Here, we report the structure and function of the O. tauri photosystem I (PSI) supercomplex in low light conditions, where it expands its photon-absorbing capacity by assembling with the light-harvesting complexes I (LHCI) and a prasinophyte-specific light-harvesting complex (Lhcp). Interestingly, nine Lhcp subunits, including one Lhcp1 monomer with a phosphorylated amino-terminal threonine and eight Lhcp2 monomers, oligomerize into three trimers and associate with PSI on the third side between Lhca6 and PsaK. While Lhcp, Lhcb (apoproteins of LHCII), and Lhca (apoproteins of LHCI) all belong to the LHC superfamily, Lhcp proteins form a separate clade with characteristics of an ancestral state of LHC proteins instead of belonging to the clades of Lhcb or Lhca. In terms of pigment composition, OtLhcp1 and OtLhcp2 each contain 14 Chl molecules (8 Chl a, 5 Chl b, and 1 Mdp) and 7 carotenoid molecules (4 Dlt, 2 Prx, and 1 Nex).

Among the three trimers associated with OtPSI, Trimers 1 and 3 are both (Lhcp2)3 homotrimers, whereas Trimer 2 is a Lhcp1(Lhcp2)2 heterotrimer. Trimers 1 and 3 bind to PSI on the PsaO and PsaK sides, respectively, while Trimer 2 assembles with PSI on the PsaL-PsaH side through Lhcp1 subunit and interacts with Lhca6 through an Lhcp2 subunit. As Trimer 1 is sandwiched between Trimers 2 and 3, it forms close contacts with both Trimers 2 and 3, and is related with them through pseudo-C2 symmetry axes at their interfaces. Among these subunits, Trimers 1 and 2 interact with each other closely and may form a stable hexameric unit. When the PSI core regions are aligned, O. tauri Trimer 1 appears to be rotated by 57 degrees and shifted by 16.1 Å in relation to the position of C. reinhardtii LHCII-1. Trimer 1 is located nearby PsaO and the closest interfacial distances between them are 7.0 Å or larger. Although Trimer 1 does not form direct interactions with PsaO, we cannot rule out the presence of unresolved lipid molecules that may mediate the interactions. In contrast, Trimer 1 appears to be poorly connected with PSI as it has Chl b molecules (Chls b608, b605, and b617 from monomer T) located at the interface with PsaO and Chl b molecules do not function as efficient bridges for EET between adjacent complexes. In the stromal layer, Chl b608T/Trimer1 faces Chl a2003PsaO, but they are separated at a relatively large Mg-Mg distance (23.9 Å). Thus, most of the energy collected by Trimer 1 is likely transferred to Trimer 2 or Trimer 3 and then pass through Chl a611-Chl a612R/Trimer2 or Chl a612W/Trimer3 to reach PSI core.

>[3x]MSALLASSFVSRVAAFKAQKVQNKSVSTTVKADIYPEFGTYPGGGESPIIPFGSEKNAEREVIHGRWAMLGVTGAWAAENGTGIPWFTAGTLCTPDDCTAVADKFPGAVAPLAPEGSGYPSFWNVLIIEIVLVGAAEAYRTGISDSPFDDGLTVGDVNPGGRFDPLGLAESGDLEELKIKELKHCRLSMFAWLGCIFQALATQEGPIANWQSHVADPVHSNVLTNAAKGFGFY> NECLVETRTTRISGRDALCVDVAGALTSDGSRLILYPCGQQVNQKWTFHSDGTVRSLGKCLATNNSKFGNLVVIYDCSKLAAEDISWDVSVGGTIMNPNYEDLALTSNKATRSTNLTMEVNTYSASQGWRVGNYVQPIIGSIVGLDDMCLEATDGNTNMWL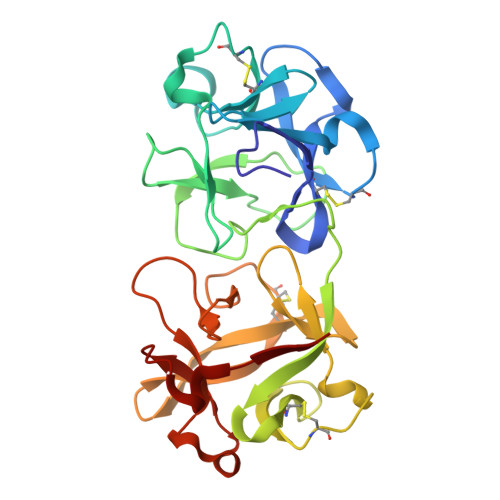EECVPNQREQSWALYSDGTIRVDDNRELCVTASSSTYDNWKVITILNCDGSNNQRWVFLADGSISTPGNQRLAMDVARSDVDLKKIILHRPHGDLNQQWVLFY>[4x]MSDWSGSVPANAENGKSTGLILKQGDTISVVAHGWVKYGRDNVEWAAP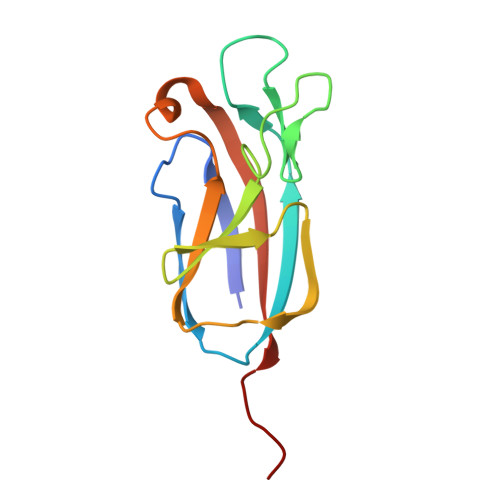DGPVPNNPQPSSIATLVAKIANKKFAIGNGVLHKTVPVDGELILLFNDVPGTFGDNSGEFQVEVIIESRYSPLK>[2x]SNADALELDTRREIYKHIVKSPGLHERQLAKELDVPLSTLVYHLHYLER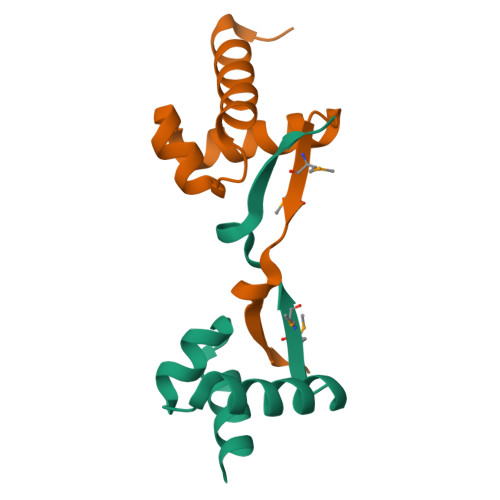RELIMMKSDERYARYYATKKLGARAKEV>MIKEAIVERIVNKLNENQKEKIGVELPSGKRIPEFPVSHLIRFKTWKSLDYVLKDPEMGFGEGYMNGDIEVEGDLEEVIKRGMTLFKDTRKFEKLFGILRHVPLFRTIRDERNVKHHYDLGNDFYRLWLDKSMTYSCAFFEDPSMSIDEAQSLKRRMIYEKLQLKEGDTLLDIGCGWGSIILESAELYNVKSVGITLSDNQYEYVKEEIKKRGLQDKVEVYKLHYVDLPKLGRKFNKVVSVGMFEHVGKENYETFFNT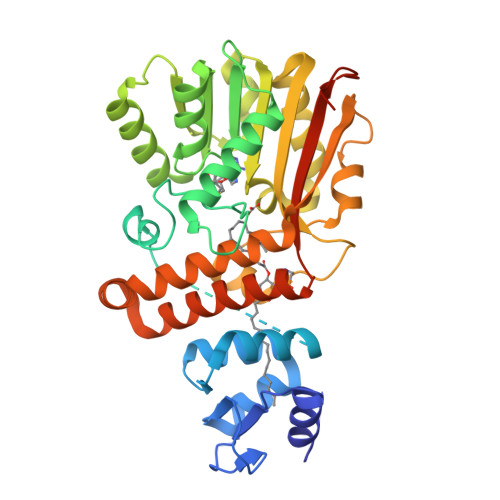VYRVMEEGGLFLLHTIGKLHPDTQSRWIRKYIFPGGYLPSISEIVESFRDMDFTLIDFDNWRMHYYWTLKKWKERFYENLDKIRNMFDDRFIRMWELYLTASAVSFLIGSNYVFQTLLSKGVKDDYPVIKREFSGVLFKEGT[2x]> MKFAVIGNPISHSLSPLMHHANFQSLNLENTYEAINVPVNQFQDIKKIISEKSIDGFNVTIPHKERIIPYLDDINEQAKS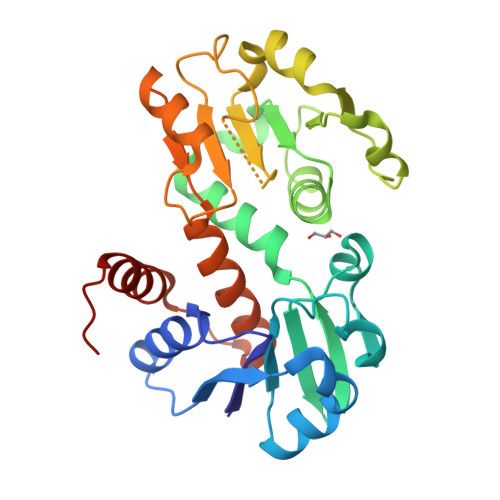VGAVNTVLVKDGKWIGYNTDGIGYVNGLKQIYEGIEDAYILILGAGGASKGIANELYKIVRPTLTVANRTMSRFNNWSLNINKINLSHAESHLDEFDIIINTTPAGMNGNTDSVISLNRLASHTLVSDIVYNPYKTPILIEAEQRGNPIYNGLDMFVHQGAESFKIWTNLEPDIKAMKNIVIQKLKGELLEHHHHHH>[2x]DYL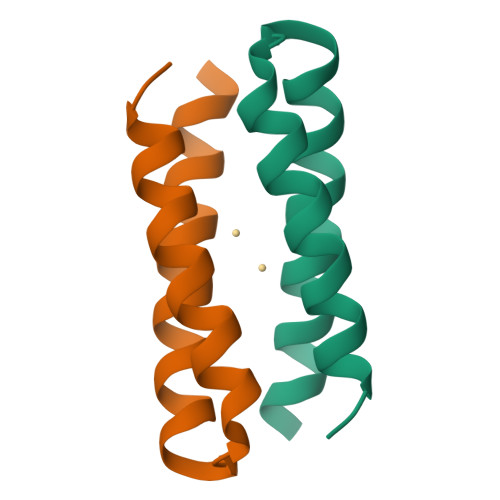RELYKLEQQAMKLYREASERVGDPVLAKILEDEEKHIEWLETI>MALALWVFGLLDLICLASANIFEYQVDAQPLRPCELQRERAFLKREDYVPQCAEDGSFQTVQCGKDGASCWCVDADGREVPGSRQPGRPAACLSFCQLQKQQILLSSYINSTATSYLPQCQDSGDYSPVQCDLRRRQCWCVDAEGMEVYGTRQQGRPARCPRSCEIRNRRLLHGVGDRSPPQCSPDGAFRPVQCKFVNTTDMMIFDLVHSYSRFPDAFVTFSSFRSRFPEVSGYCYCADSQGRELAETGLELLLDEIYDTIFAGLDLASTFAETTLYRILQRRFLAVQLVISGRFRCPTKCEVERFAATSFRHPYVPSCHPDGEYQAAQCQQGGPCWCVDSRGQEIPGTRQRGEPPSCAEDQSCPSERRRAFSRLRFGPSGYFSRRSLLLAPEEGPVSQRFARFTASCPPSIKELFLDSGIFQPMLQGRDTRFVAPESLKEAIRGLFPSRELARLALQFTTNAKRLQQNLFGGRFLVKVGQFNLSGALGTRGTFNFSHFFQQLGLPGFQDGRALADLAKPLSVGLNSNPASEAPKASKIDVALRKPVVGSFGFEVNLQENQNALQFLSSFLELPEFLLFLQHAISVPEDIARDLGDVMEMVFSSQGCGQAPGSLFVPACTAEGSYEEVQCFAGDCWCVDAQGRELAGSRVRGGRPRCPTECEKQRARMQSLLGSQPAGSSLFVPACTSKGNFLPVQCFNSECYCVDTEGQPIPGTRSALGEPKKCPSPCQLQAERAFLGTVRTLVSNPSTLPALSSIYIPQCSASGQWSPVQCDGPPEQAFEWYERWEAQNSAGQALTPAELLMKIMSYREAASRNFRLFIQNLYEAGQQGIFPGLARYSSFQDVPVSVLEGNQTQPGGNVFLEPYLFWQILNGQLDRYPGPYSDFSAPLAHFDLRSCWCVDEAGQKLEGTRNEPNKVPACPGSCEEVKLRVLQFIREAEEIVTYSNSSRFPLGESFLAAKGIRLTDEELAFPPLSPSRETFLEKFLSGSDYAIRLAAQSTFDFYQRRLVTLAESPRAPSPVWSSAYLPQCDAFGGWEPVQCHAATGHCWCVDGKGEYVPTSLTARSRQIPQCPTSCERLRASGLLSSWKQAGVQAEPSPKDLFIPTCLETGEFARLQASEAGTWCVDPASGEGVPPGTNSSAQCPSLCEVLQSGVPSRRTSPGYSPACRAEDGGFSPVQCDPAQGSCWCVLGSGEEVPGTRVAGSQPACESPQCPLPFSVADVAGGAILCERASGLGAAAGQRCQLRCSQGYRSAFPPEPLLCSVQRRRWESRPPQPRACQRPQFWQTLQTQAQFQLLLPLGKVCSADYSGLLLAFQVFLLDELTARGFCQIQVKTAGTPVSIPVCDDSSVKVECLSRERLGVNITWKLQLVDAPPASLPDLQDVEEALAGKYLAGRFADLIQSGTFQLHLDSKTFSADTSIRFLQGDRFGTSPRTQFGCLEGFGRVVAASDASQDALGCVKCPEGSYFQDEQCIPCPAGFYQEQAGSLACVPCPEGRTTVYAGAFSQTHCVTDCQKNEVGLQCDQDSQYRASQRDRTSGKAFCVDGEGRRLPWTEAEAPLVDAQCLVMRKFEKLPESKVIFSADVAVMVRSEVPGSESSLMQCLADCALDEACGFLTVSTAGSEVSCDFYAWASDSIACTTSGRSEDALGTSQATSFGSLQCQVKVRSREGDPLAVYLKKGQEFTITGQKRFEQTGFQSALSGMYSPVTFSASGASLAEVHLFCLLACDHDSCCDGFILVQVQGGPLLCGLLSSPDVLLCHVRDWRDPAEAQANASCPGVTYDQDSRQVTLRLGGQEIRGLTPLEGTQDTLTSFQQVYLWKDSDMGSRSESMGCRRDTEPRPASPSETDLTTGLFSPVDLIQVIVDGNVSLPSQQHWLFKHLFSLQQANLWCLSRCAGEPSFCQLAEVTDSEPLYFTCTLYPEAQVCDDILESSPKGCRLILPRRPSALYRKKVVLQDRVKNFYNRLPFQKLTGISIRNKVPMSDKSISSGFFECERLCDMDPCCTGFGFLNVSQLKGGEVTCLTLNSLGLQTCSEEYGGVWRILDCGSPDTEVRTYPFGWYQKPVSPSDAPSFCPSVALPALTENVALDSWQSLALSSVIVDPSIRNFDVAHISTAAVGNFSAARDRCLWECSRHQDCLVTTLQTQPGAVRCMFYADTQSCTHSLQAQNCRLLLHEEATYIYRKPNIPLPGFGTSSPSVPIATHGQLLGRSQAIQVGTSWKPVDQFLGVPYAAPPLGEKRFRAPEHLNWTGSWEATKPRARCWQPGIRTPTPPGVSEDCLYLNVFVPQNMAPNASVLVFFHNAAEGKGSGDRPAVDGSFLAAVGNLIVVTASYRTGIFGFLSSGSSELSGNWGLLDQVVALTWVQTHIQAFGGDPRRVTLAADRGGADIASIHLVTTRAANSRLFRRAVLMGGSALSPAAVIRPERARQQAAALAKEVGCPSSSVQEMVSCLRQEPARILNDAQTKLLAVSGPFHYWGPVVDGQYLRETPARVLQRAPRVKVDLLIGSSQDDGLINRAKAVKQFEESQGRTSSKTAFSQALQNSLGGEAADAGVQAAATWYYSLEHDSDDXASFSRALEQATRDYFIICPVIDMASHWARTVRGNVFMYHAPESYSHSSLELLTDVLYAFGLPFYPAYEGQFTLEEKSLSLKIMQYFSNFIRSGNPNYPHEFSRRAPEFAAPWPDFVPRDGAESYKELSVLLPNRQGLKKADCSFWSKYIQSLKASADETKDGPSADSEEEDQPAGSGLTEDLLGLPELASKTYSK[2x]

Thyroid hormones T3 (tri-iodothyronine) and T4 (tetra-iodothyronine or thyroxine) are essential regulators of metabolism, development, and growth in all vertebrates and some invertebrates. T3 and T4 are formed from the precursor thyroglobulin (TG), a ~660-kDa homodimer specific to the follicular lumen of the thyroid gland. T3 is formed when the mono-iodinated phenolic ring of a donor tyrosine is transferred to a di-iodinated acceptor tyrosine; T4 is formed when the donor tyrosine phenolic ring is also di-iodinated. In addition to being the site of hormone formation, TG functions as a reservoir for thyroid hormone storage until it is trafficked back into the thyrocyte and degraded in the lysosome, liberating T3 and T4 for secretion into the bloodstream.

Here we report a ~3.3-Å cryo-EM structure of native bovine TG with nascent thyroid hormone present at the predicted hormonogenic site B. A cryo-EM reconstruction was obtained with a ~3.3 Å overall resolution and a ~2.8 Å local resolution over a substantial, presumably more rigid part of the complex, sufficient for building an atomic model. The structure is essentially identical to that of recombinant human TG6, including conservation of multiple glycosylation sites. Close agreement between the density map and the model confirms that the acceptor tyrosine is 3,5-di-iodinated (top), as required for thyroid hormone formation. The map for the transferred donor phenolic group appears ambiguous regarding iodination state (top), as might be expected if the map includes a mixture of donor mono- and di-iodination states (corresponding to nascent T3 and T4, respectively), heterogeneity in the orientation of the donor aromatic ring, or both. Tandem mass spectrometry analysis (LC-MS/MS) confirmed that there was a mixture of nascent T3 and T4 at position 2573 in the TG sample. At the predicted donor site (bottom), the map fits a dehyrdroalanine residue but does not appear to accommodate the original tyrosine aromatic side chain, whereas the map makes a good fit to other side chains of the loop containing the donor site (pale blue), including the aromatic side chain of the immediately adjacent residue F2439. The nascent thyroid hormone at hormonogenic site B is accompanied by a substantial alteration of neighboring structural elements as compared with pre-hormonogenic human TG6. The helix-loop-helix motif formed by residues 2515–2548 (dark gray-blue) is substantially reorganized, rotating F2539 (green) by ~80° and displacing it by ~9 Å from its initial position. This rearrangement moves the acceptor tyrosine (red) away from its close apposition to F2576 (gold), flips the residual donor site far away, and packs the double-ringed reaction product into an interior pocket bounded by α-helices.> SLRLLDHRALVCSQPGLNCTVKNSTCLDDSWIHPRNLTPSSPKDLQIQLHFAHTQQGDLFPVAHIEWTLQTDASILYLEGAELSVLQLNTNERLCVRFEFLSKLRHHHRRWRFTFSHFVVDPDQEYEVTVHHLPKPIPDGDPNHQSKNFLVPDCEHARMKVTTPCMSSGSLWDPNITVETLEAHQLRVSFTLWNESTHYQILLTSFPHMENHSCFEHMHHIP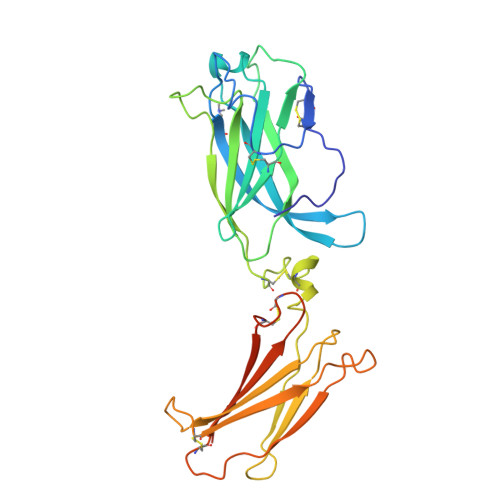APRPEEFHQRSNVTLTLRNLKGCCRHQVQIQPFFSSCLNDCLRHSATVSCPEMPDTPEPIPDYM>[4x]GMIRLSNENTIFFMDKENVPIASCQSGDTVIFETKDCFSDQITNEEQALTSIDFNRVNPATGPLYVEGARRGDMLEIEILDIKVGKQGVMTAAPGLGALGESLNSPTTKLFPIEGDDVVYSTGLRLPLQPMIGVIGTAPPGEPINNGTPGPHGGNLDTKDIKPGTTVYLPVEVDGALLALGDLHAAMGDGEILICGVEIAGTVTLKVNVKKERMFPLPALKTDTHFMTIASAETLD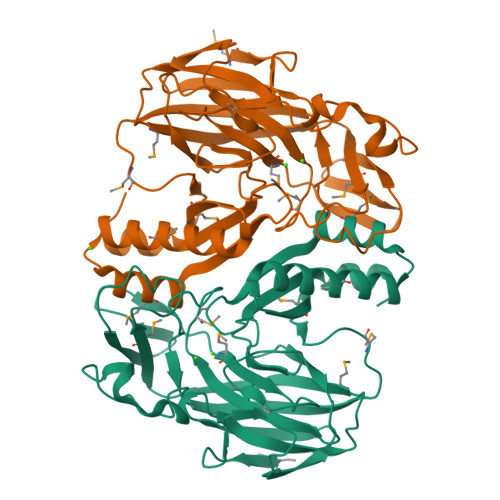AAAVQATKNMATFLANRTALSIEEAGMLLSGAGDLYVSQIVNPLKTARFSLALHYFEKLGVDLCN>[2x]STHFDVIVVGAGSMGMAAGYQLAKQGVKTLLVDAFDPPHTNGSHHGDTRIIRHAYGEGREYVPLALRSQELWYELEKETHHKIFTKTGVLVFGPKGESAFVAETMEAAKEHSLTVDLLEGDEINKRWPGITVPENYNAIFEPNSGVLFSENCIRAYRELAEARGAKVLTHTRVEDFDISPDSVKIETANGSYT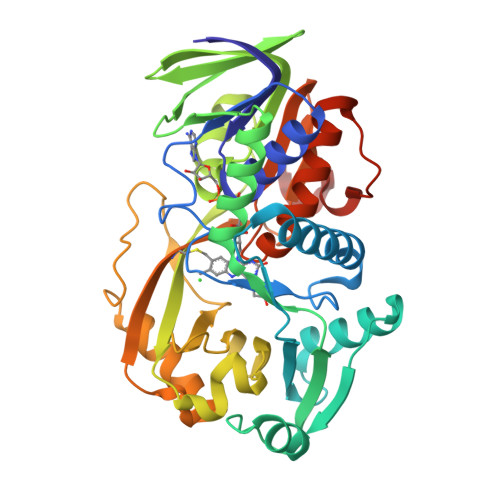ADKLIVSMGAWNSKLLSKLNLDIPLQPYRQVVGFFESDESKYSNDIDFPGFMVEVPNGIYYGFPSFGGCGLKLGYHTFGQKIDPDTINREFGVYPEDESNLRAFLEEYMPGANGELKRGAVCMYTKTLDEHFIIDLHPEHSNVVIAAGFSGHGFKFSSGVGEVLSQLALTGKTEHDISIFSINRPALKESLQKTTI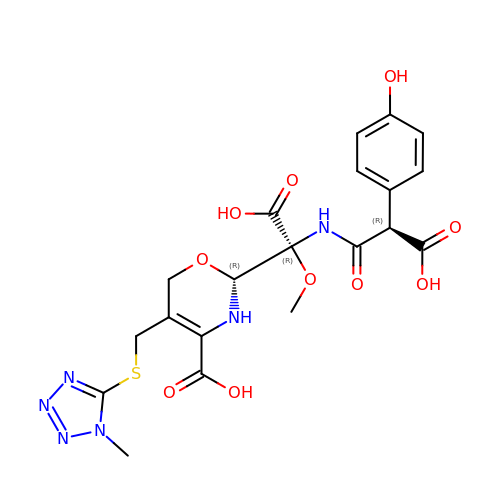(2R)-2-[(R)-carboxy{[(2R)-2-carboxy-2-(4-hydroxyphenyl)acetyl]amino}methoxymethyl]-5-{[(1-methyl-1H-tetrazol-5-yl)sulfanyl]methyl}-3,6-dihydro-2H-1,3-oxazine-4-carboxylic acid | C20 H22 N6 O10 S | BNVHAJAUCCPJNC-WYAVIUHXSA-N> MKPSIVAKLEALHERHEEVQALLGDAQTIADQERFRALSREYAQLSDVSRCFTDWQQVQEDIETAQMMLDDPEMREMAQDELREAKEKSEQLEQQLQVLLLPKDPDDERNAFLEVRAGTGGDEAALFAGDLFRMYSRYAEARRWRVEIMSASEGEHGGYKEIIAKISGDGVYGRLKFESGGHRVQRVPATESQGRIHTSACTVAVMPELPDAELPDVNPADLRIDTFRSSGAGGQHVNTTDSAIRITHLPTGIVVECQDERSQHKNKAKALSVLGARIHAAEMAKRQQAEASTRRNL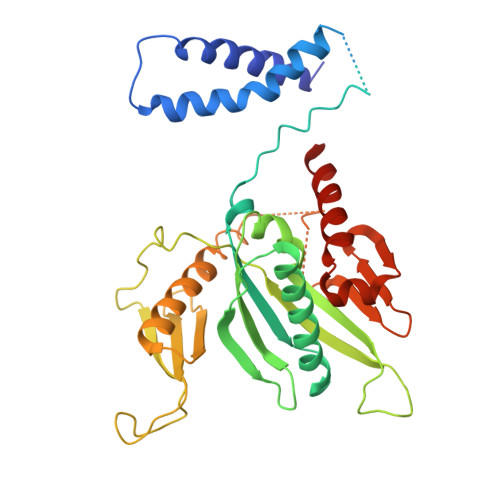LGSGDRSDRNRTYNFPQGRVTDHRINLTLYRLDEVMEGKLDMLIEPIIQEHQADQLAALSEQE>GSAAPGLLRQELSCPLCLQLFDAPVTAECGHSFCRACLIRVAGEPAADGTVACPCCQAPTRPQALSTNLQLSRLVEGLAQVPQGHCEEHLDPLSIYCEQDRTLVCGVCASLGSHRGHRLLPAAEAQARLKTQLPQQKMQLQEACMRKEKTVAVLEHQLVEVEETVRQFRGAVGEQLGKMRMFLAALESSLDREAERVRGDAGVALRRELSSLNSYLEQLRQMEKVLEEVADKPQTEFLMKFCLVTSRLQKILSESPPPARLDIQLPVISDDFKFQVWKKMFRALMPALEELTFDPSSAHPSLVVSSSGRRVECSDQKAPPAGEDTRQFDKAVAVVAQQLLSQGEHYWEVEVGDKPRWALGVMAADASRRGRLHAVPSQGLWLLGLRDGKILEAHVEAKEPRALRTPERPPARIGLYLSFADGVLAFYDASNPDVLTPIFSFHERLPGPVYPIFDVCWHDKGKNAQPLLLVGPEQEQA[2x]

Tripartite motif-containing protein (TRIM)72 (mitsugumin 53; MG53) has been determined to rapidly nucleate vesicles at the site of membrane damage, but the underlying molecular mechanisms remain poorly understood. Here we present the structure of Mus musculus TRIM72, a complete model of a TRIM E3 ubiquitin ligase. TRIM72 is a member of the class IV TRIM proteins, which is the largest subtype among the 11 groups of TRIM proteins. Its domain organization includes an RBCC domain followed by a PRY motif associated with a SPRY domain identified in splA kinase and ryanodine receptors (PRYSPRY) domain.

To obtain a high-resolution model, numerous constructs were generated, purified and crystallized; however, most of them diffracted poorly. After introducing point mutations and deletions, we were finally able to resolve molecular models of mouse TRIM72, including RING-deleted (ΔRING, 2.75 Å; the highest resolution is in parentheses), full-length (FL, 4.6 Å) and wild-type (WT, 7.1 Å) TRIM72. TRIM72 is a tight dimer, as determined by size exclusion chromatography (SEC) coupled with multiangle light scattering (SEC–MALS), and its overall shape was determined to be elongated in solution by SEC coupled with small-angle X-ray scattering (SEC–SAXS). The overall structure of the TRIM72 dimer has an elongated shape. The coiled-coil domains (CCDs) form the main scaffold of an antiparallel dimer with a length of approximately 17 nm.6-O-CYCLOHEXYLMETHYL GUANINE | C12 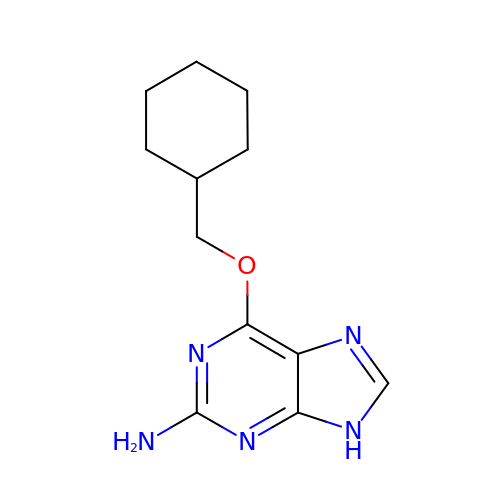H17 N5 O | MWGXGTJJAOZBNW-UHFFFAOYSA-N>MGSDKIHHHHHHENLYFQGMIKVNVMYPYTEGARFDHAYY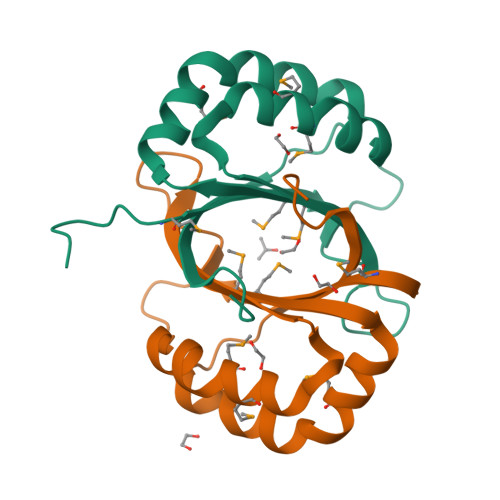CDRHMPMVKARLGSACAYYTVEKGLAGSASGAPPAFVAMCAFICDSAENFYAAMYYHGAEILGDIANYTDIAPVLQISEVVVERSDR[2x]>MGSSHHHHHHSSGLVPRGSHMASATASRGASQAGAPQGRVPEARPNSMVVEHPEFLKAGKEPGLQIWRVEKFDLVPVPTNLYGDFFTGDAYVILKTVQLRNGNLQYDLHYWLGNECSQDESGAAAIFTVQLDDYLNGRAVQHREVQGFESATFLGYFKSGLKYKKGGVASGFKHVVPNEVVVQRLFQVKGRRVVRATEVPVSWESFKNGDCFILDLGNNIHQWCGSNSNRYERLKATQVSKGIRDNERSGRARVHVSEEGTEPEAMLQVLGPKPALPAGTEDTAKEDAANRKLAKLYKVSNGAGTMSVSLVADENPFAQGALKSEDCFILDHGKDGKIFVWKGKQANTEERKAALKTASDFITKMDYPKQTQVSVLPEGGETPLFKQFFKNWRDPDQTDGLGLSYLSSHIANVERVPFDAATLHTSTAMAAQHGMDDDGTGQKQIWRIEGSNKVPVDPATYGQFYGGDSYIILYNYRHGGRQGQIIYNWQGAQSTQDEVAASAILTAQLDEELGGTPVQSRVVQGKEPAHLMSLFGGKPMIIYKGGTSREGGQTAPAST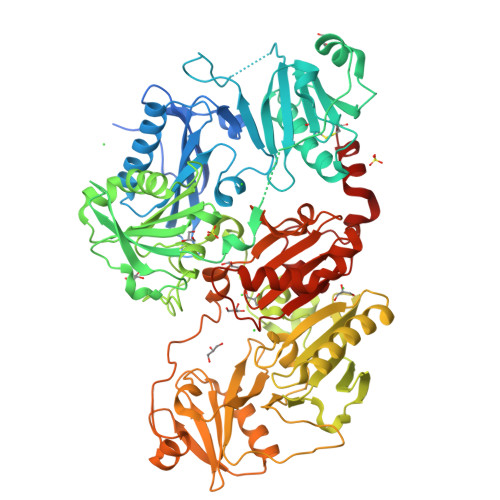RLFQVRANSAGATRAVEVLPKAGALNSNDAFVLKTPSAAYLWVGTGASEAEKTGAQELLRVLRAQPVQVAEGSEPDGFWEALGGKAAYRTSPRLKDKKMDAHPPRLFACSNKIGRFVIEEVPGELMQEDLATDDVMLLDTWDQVFVWVGKDSQEEEKTEALTSAKRYIETDPANRDRRTPITVVKQGFEPPSFVGWFLGWDDDYWSVDPLDRAMAELAA[2x]> AA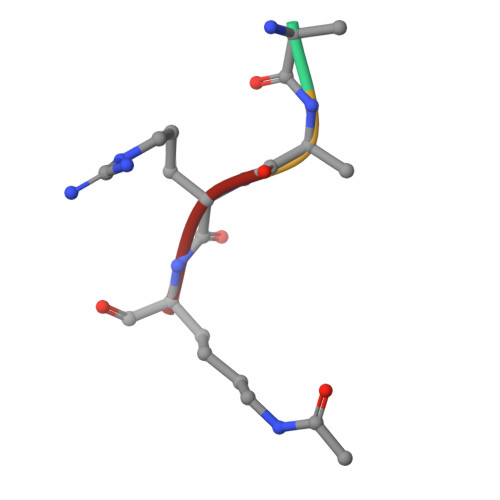RK3-[(2S)-2-{[(4-methylphenyl)sulfonyl]amino}-3-oxo-3-piperidin-1-ylpropyl]benzenecarboximidamide | C22 H28 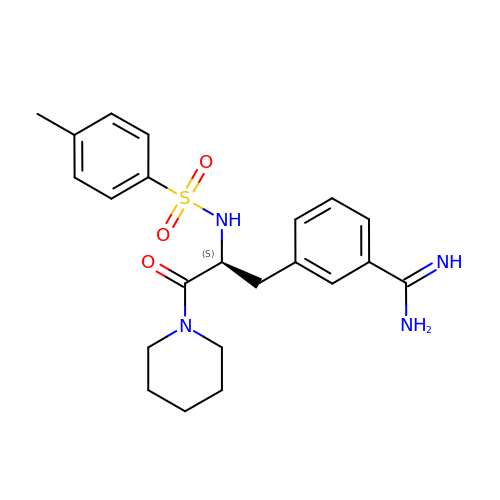N4 O3 S | RNNMXTSTLVYYQG-FQEVSTJZSA-N>MKYPRTCFFSALLLFYSMIAAINFASAQTSEQFEWNKLPVKAMLLTVPHPEDVPEFCRFIKEVLPKEGVNTLVLRIRYNYKFKSHPELAGERAISEQQLKQIVQTCKEAKIRFIPKMNLLGHQSDRDHIDPLLAKYPQFDESPDYNPPVPWKDAGPFDFYCKSLCPSHPDLLKTIFPLMDELIDVCGADAFHVGLDEVWILGYEKCPRCGGRDKAALFAEYATKLHDHLKEKKCQMWMWSDRLIDGKTTNLLGWQASMNATFRA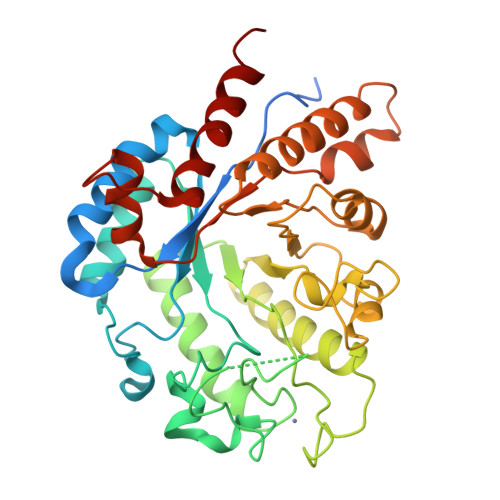IDLIPTDIMICDWKYESAPPTPGYFAIKGFNVLPSSCSNSEVALAQLAQVRLARKDGTRAPWAVTLAERMQGVFVTMWEDSKEFIDAYYGRNGKKLPSAETFKAVFAQIRKEEVMN[5x]>ARKCSLTGKWTNNLGSIMTIRAVNSRGEFTGTYLTAVADNPGNITLSPLLGIQHKRASQPTFGFTVHWNFSESTTVFTGQCFID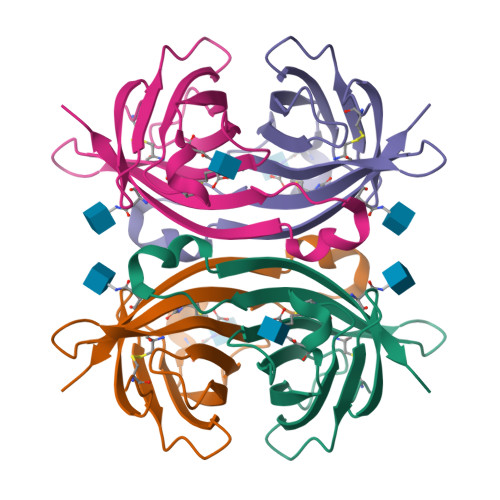RNGKEVLKTMWLLRSSVNDISYDWKATRVGYNNFTRLSTVEE[2x]> GTSSMADIGSEPFSLKTHRFNPFAYVDFGNDVVLTEDILSQIDTRLKGHGMVAS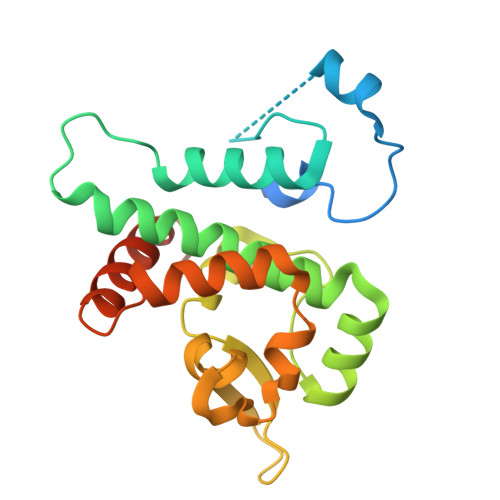GGDFSTQIFGLAKLVFPERPNEKDPFFSNQARNLFVINCNIYRDLMWTKKGLEFVKRKKIIMPETPTMFFIGSMASGINLIDEDTNMEKVVSLMEFFGGEEDKSGDNLRVLSPATRNMWNSFKTMGGARETYSSVQGVYTSAFAPYNNAMIRNFTS Protoglobin (Pgb) is a recently discovered haem-protein with distinct structural and functional features that make it unique within the globin superfamily. The MaPgb* structure can be considered as an expanded version of the 3/3 helical sandwich typical of “classical” globins (i.e. Mb), with an additional N-terminal extension, built by a 20-residue loop, followed by the Z-helix, which precedes the globin-fold conserved A-helix. Residues belonging to the Z-helix contribute to formation of the Pgb homodimer, which is centered on the intermolecular four-helix bundle built by the G- and H-helices of the two subunits. Thus, in Pgb the access of diatomic ligands, such as O2, CO, and NO, to the haem is granted by two orthogonal apolar tunnels that reach the haem distal region from entry sites at the B/G and B/E helix interfaces.

The sites of MaPgb*(III) mutations (Trp(60)B9Ala, Tyr(61)B10Ala, Phe(93)E11Leu, Leu(142)G4Ala, and Ile(149)G11Phe) are located in the surroundings of the haem, or along the two tunnels; the mutations were designed to evaluate the (structural) impact of the selected residues on the stabilization of the haem-Fe(III)-bound ligand and on the reshaping of the haem distal cavity/tunnel system. The other two mutations considered, Leu(142)G4Ala, localized at the proximal site just on top of His(120)F8, and Ile(149)G11Phe, adjacent to Trp(60)B9 in tunnel 1, do not produce any significant deviation in the overall conformation of the distal site and in the cyanide binding mode relative to the MaPgb*(III)-cyanide structure. off for cyanide dissociation from cyanide-bound MaPgb*(III) and Leu(142)G4Ala and from the Ile(149)G11Phe ferric mutants, all characterized by ligand stabilization through two H-bonds (to Trp(60)B9 and Tyr(61)B10), are lower than those reported for ligand dissociation from the Tyr(61)B10Ala and Trp(60)B9Ala MaPgb*(III)-cyanide species, characterized by ligand stabilization through one H-bond. Overall, the single mutations do not affect significantly the tertiary structure of the mutated proteins, which are always closely similar in their backbone to that of MaPgb*(III)-cyanide, displaying rms deviation values which range between 0.17 Å and 0.49 Å, calculated for 190 Cα atom pairs.

>MSVEKIPGYTYGETENRAPFNLEDLKLLKEAVMFTAEDEEYIQKAGEVLEDQVEEILDTWYGFVGSHPHLLYYFTSPDGTPNEKYLAAVRKRFSRWILDTSNRSYDQAWLDYQYEIGLRHHRTKKNQTDNVESVPNIGYRYLVAFIYPFTATMKPFLARKGHTPEEVEKMYQAWFKATTLQVALWSYPYVKYGDF[3x]>MIKQRTLK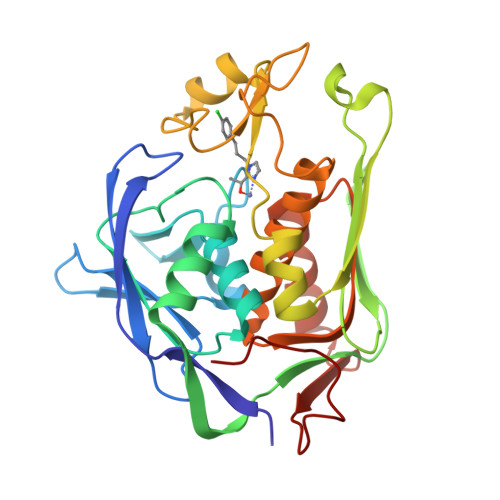NIIRATGVGLHSGEKVYLTLKPAPVDTGIVFSRTDLDPVVEIPARAENVGETTMSTTLVKGDVKVDTVEHLLSAMAGLGIDNAYVELSASEVPIMDGSAGPFVFLIQSAGLQEQEAAKKFIRIKREVSVEEGDKRAVFVPFDGFKVSFEIDFDHPVFRGRTQQASVDFSSTSFVKEVSRARTFGFMRDIEYLRSQNLALGGSVENAIVVDENRVLNEDGLRYEDEFVKHKILDAIGDLYLLGNSLIGEFRGFKSGHALNNQLLRTLIADKDAWEVVTFEDARTAPISYMRP[2x]> SGVDDDMACHKIPVEADFLYAYS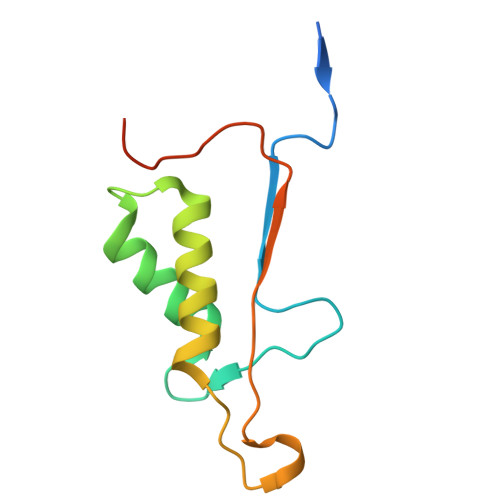TAPGYYSWRNSKDGSWFIQSLCAMLKQYADKLEFMHILTRVNRKVATEFESFSFDATFHAKKQIPCIVSMLTKELYFYHLEHHHHHH Ctf18-RFC belongs to the RFC family of AAA+ ATPase clamp loaders, which are involved in the loading and unloading of clamps onto dsDNA. Compared to other clamp loaders, Ctf18-RFC contains two additional subunits, Ctf8 and Dcc1, which bind to the C-terminus of Ctf18 to form the Ctf18-1-8 module. Mutations in Ctf18 that disrupt formation of this Ctf18-1-8 module result in similar but not identical phenotypes as entire deletions of Ctf18 (29,30), suggesting that this module is critical for at least some of the specialized functions of Ctf18-RFC. It has been shown that the Ctf18-1-8 module binds the N-terminal catalytic domain of Pol2 (30,31), the largest subunit of the leading strand Pol ϵ, and that this interaction increases the clamp loader activity of Ctf18-RFC.

We therefore used cryo-EM to solve the structure of the Ctf18-1-8 module in complex with the complete catalytic domain of Pol2 (residues 1–1192, henceforth Pol2CAT) to 4.2 Å resolution. This is the largest Pol ϵ/Ctf18-RFC complex that can be structurally analyzed due to the large-scale flexibility of both Pol ϵ and Ctf18-RFC. Our structure reveals that the complete Ctf18-1-8/Pol2CAT complex has a large interface burying an area of 1363 Å2, which is more than double the 612 Å2 area buried in the minimal complex. Dcc1WH3 interacts with Pol2EXO as previously observed, but this interface is now further stabilized by the Pol2 fingers subdomain (Pol2FINGERS). Furthermore, entirely new interactions are formed by the Ctf18-1-8 triple-barrel domain (TBD), which has rotated towards the polymerase to interact with Pol2EXO and the Pol2 thumb (Pol2THUMB) subdomain in two discontinuous interaction patches. Unlike the Dcc1WH3-Pol2EXO and TBD-Pol2THUMB interfaces, which are mostly electrostatic in nature and show few specific interactions, the TBD-Pol2EXO patch is well-ordered and displays hydrophobic and backbone interactions involving highly-conserved amino acids. This interface centers on an extension of the Pol2EXO beta-sheet into the upper beta-barrel of Ctf18-1-8, via a beta-strand formed by the conserved 730V(R/K)(R/K)732 motif in Ctf18, resulting in a distorted four-protein anti-parallel beta-sheet. Comparing our DNA-free structure of Pol2CAT with the crystal structure of the DNA- and nucleotide-trapped Pol2CAT shows movements of the Pol2THUMB, Pol2PALM and Pol2FINGERS subdomains that are characteristic of B-family DNA polymerases. The large interface suggested that this might be a stable interaction, and so we measured the affinity between Ctf18-1-8 and Pol2CAT by isothermal titration calorimetry. This showed that Ctf18-1-8 forms a tight complex with Pol2CAT with a KD of 40 nM, approximately 30-fold stronger than the 1.3 μM KD measured for the truncated Pol2(1–528) construct.

> MKHHHHHHSAGLEVLFQGPGTGSEFELMMFGKKKNNGGSSTARYSAGNKYNTLSNNYALSAQQLLNASKIDDIDSMMGFERYVPPQYNGRFDAKDIDQIPGRVGWLTNMHATLVSQETLSSGSNGGGNSNDGERVTTNQGISGVDFYFLDEEGGSFKSTVVYDPYFFIACNDESRVNDVEELVKKYLESCLKSLQIIRKEDLTMDNHLLGLQKTLIKLSFVNSNQLFEARKLLRPILQDNANNNVQRNIYNVAANGSEKVDAKHLIEDIREYDVPYHVRVSIDKDIRVGKWYKVTQQGFIEDTRKIAFADPVVMAFAIATTKPPLKFPDSAVDQIMMISYMIDGEGFLITNREIISEDIEDFEYTPKPEYPGFFTIFNENDEVALLQRFFEHIRDVRPTVISTFNGDFFDWPFIHNRSKIHGLDMFDEIGFAPDAEGEYKSSYCSHMDCFRWVKRDSYLPQGSQGLKAVTQSKLGYNPIELDPELMTPYAFEKPQHLSEYSVSDAVATYYLYMKYVHPFIFSLCTIIPLNPDETLRKGTGTLCEMLLMVQAYQHNILLPNKHTDPIERFYDGHLLESETYVGGHVESLEAGVFRSDLKNEFKIDPSAIDELLQELPEALKFSVEVENKSSVDKVTNFEEIKNQITQKLLELKENNIRNELPLIYHVDVASMYPNIMTTNRLQPDSIKAERDCASCDFNRPGKTCARKLKWAWRGEFFPSKMDEYNMIKRALQNETFPNKNKFSKKKVLTFDELSYADQVIHIKKRLTEYSRKVYHRVKVSEIVEREAIVCQRENPFYVDTVKSFRDRRYEFKGLAKTWKGNLSKIDPSDKHARDEAKKMIVLYDSLQLAHKVILNSFYGYVMRKGSRWYSMEMAGITCLTGATIIQMARALVERVGRPLELDTDGIWCILPKSFPETYFFTLENGKKLYLSYPCSMLNYRVHQKFTNHQYQELKDPLNYIYETHSENTIFFEVDGPYKAMILPSSKEEGKGIKKRYAVFNEDGSLAELKGFELKRRGELQLIKNFQSDIFKVFLEGDTLEGCYSAVASVCNRWLDVLDSHGLMLEDEDLVSLICENRSMSKTLKEYEGQKSTSITTARRLGDFLGEDMVKDKGLQCKYIISSKPFNAPVTERAIPVAIFSADIPIKRSFLRRWTLDPSLEDLDIRTIIDWGYYRERLGSAIQKIITIPAALQGVSNPVPRVEHPDWLKRKIAT;> MSINLHSAPEYDPSYKLIQLTPELLDIIQDPVQNHQLRFKSLDKDKSEVVLCSHDKTWVLKQRKHSNTVLLMREFVPEQPITFDETLLFGLSKPYMDVVGFAKTESEFETRETHGELNLNSVPIYNGELDFSDKIMKRSSTKVIGTLEELLENSPCSALEGISKWHKIGGSVKDGVLCILSQDFLFKALHVLLMSAMAESLDLQHLNVEDTHHAVGKDIEDEFNPYTREIIETVLNKFAVQEQEAENNTWRLRIPFIAQWYGIQALRKYVSGISMPIDEFLIKWKSLFPPFFPCDIDIDMLRGYHFKPTDKTVQYIAKSTLPMDPKERFKVLFRLQSQWDLEDIKPLIEELNSRGMKIDSFIMKYARRKRLGKKTVVTSR;> MPSVDIDASQWQKLTQSREKQTTVITPLGMMMLEIQGELELPKDFASLARRDSPNEGRFSEQDGETLIRFGSLQIDGERATLFVGKKQRLLGKVTKLDVPMGIMHFNSKDNKVELVDVMKYKVIFKDRPLPIM;> GAMGNQTVKIWVKYNEGFSNAVRKNVTWNNLWE>[2x]MAHHHHHHMIREILKMG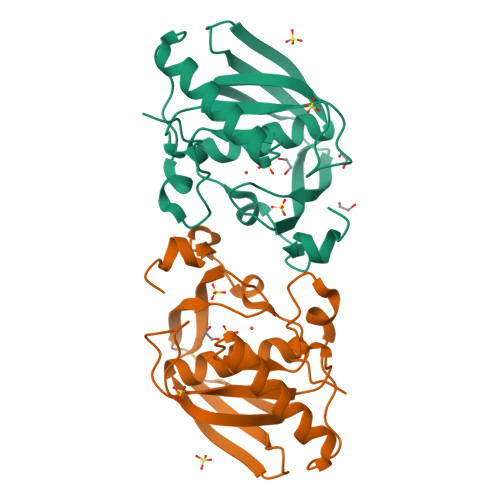DPRLLEVAKPVAQFDTPELHEIVADMFETMHHANGAGLAAPQIGIGLQIIIFGFGSNNRYPDAPPVPETVLINPKLEYMPPDMEEGWEGCLSVPGMRGVVSRYAKVRYSGYDQFGAKIDRVAEGFHARVVQHEYDHLIGKLYPMRITDFTRFGFTEVLFPGLDPTDDD>[2x]MVEQIKDKLGRPIRDLRLSVTDRCNFRCDYCMPKEVFGDDFVFLPKNELLTFDEMARIAKVYAELGVKKIRITGGEPLMRRDLDVLIAKLNQIDGIEDIGLTTNGLLLKKHGQKLYDAGLRRINVSLDAIDDTLFQSINNRNIKATTILEQIDYATSIGLNVKVNVVIQKGINDDQIIPMLEYFKDKHIEIRFIEFMDVGNDNGWDFSKVVTKDEMLTM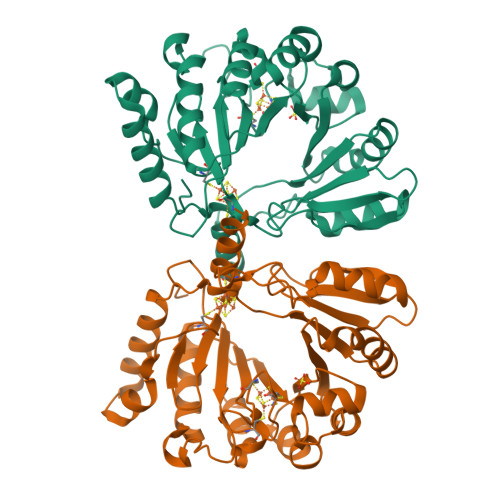IEQHFEIDPVEPKYFGEVAKYYRHKDNGVQFGLITSVSQSFCSTCTRARLSSDGKFYGCLFATVDGFNVKAFIRSGVTDEELKEQFKALWQIRDDRYSDERTAQTVANRQRKKINMNYIGG> MRFRPFTEEDLDRLNRLAGKRPVSLGALRFFARTGHSFLAEEGEEPMGFALAQAVWQGEATTVLVTRIEGRSVEALRGLLRAVVKSAYDAGVYEVALHLDPERK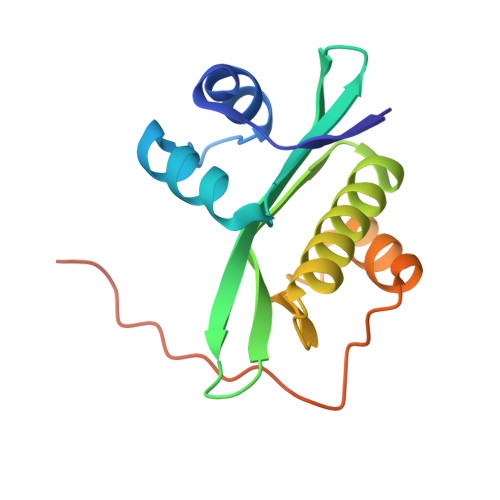ELEEALKAEGFALGPLVLAVRVLGSRGARGETRGVLE>[18x]GIPPKIEALPSDISI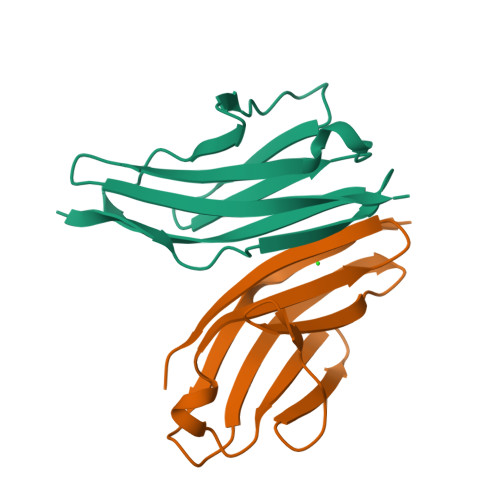DEGKVLTVACAFTGEPTPEVTWSCGGRKIHSQEQGRFHIENTDDLTTLIIMDVQKQDGGLYTLSLGNEFGSDSATVNIHIRS;>[18x]SSAPRFLTRPKAFVVSVGKDATLSCQIVGNPTPQVSWEKDQQPVAAGARFRLAQDGDLYRLTILDLALGDSGQYVCRARNAIGEAFAAVGLQV> MALPLLNYAPKSQNVRVEGYEIGSEEKPVVFTTENILSSSDMDNLIEAAYRQIFFHAFKWDREKVLESQLRNGQITVRDFVRGLLLSNTFRNSFYEKNSNYRFVEHCVQKILGRDVYSEREKIAW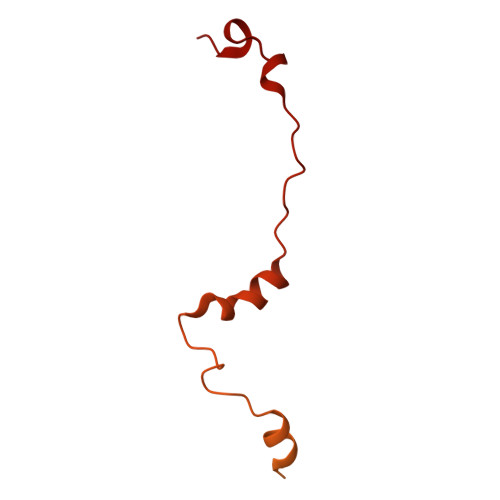SIVVATKGYQGLIDDLLNSDEYLNNFGYDTVPYQRRRNLPGREAGELPFNIKSPRYDAYHRRQLGFPQIVWQNEVRRFIPQEKKLTAGNPMNFLGMARSINPAANTIPKVSAQNINIEASVPRR>[2x]MPIITDVYAREVLDSRGNPTVEVEVLTESGAFGRALVPSGASTGEHEAVELRDGDKSRYLGKGVTKAVENVNEIIAPEIIEGEFSVLDQVSIDKMMIALDGTPNKGKLGANAILGVSIAVARAAADLLGQPLYKYLGGFNGKQLPVPMMNIVNGGSHSDAPIAFQEFMILPVGATTFKESLRWGTEIFHNLKSILSKRGLETAVGDEGGFAPKFEGTEDAVETIIQAIEAAGYKPGEEVFLGFDCASSEFYENGVYDYSKFEGEHGAKRTAAEQVDYLEQLVDKYPIITIEDGMDENDWDGWKQLTERIGDRVQLVGDDLFVTNTEILAKGIENGIGNSILIKVNQIGTLTETFDAIEMAQKAGYTAVVSHRSGETEDTTIADIAVATNAGQIKTGSLSRTDRIAKYNQLLRIEDELFETAKYDGIKSFYNLDKLEHHHHHH

Enolase is a glycolytic enzyme that requires a divalent metal ion (optimally Mg2+) bound in the active site to catalyze the dehydration of 2-phosphoglycerate (2-PG) to phosphoenolpyruvate (PEP), as well as the reverse reaction in the gluconeogenesis pathway. Interestingly, enolase has been identified on the cell surface of S. aureus, enhancing the staphylokinase activation of plasminogen. The Sa_enolase monomer has two distinct domains, a small N-terminal domain (residues 1–137) and a large C-terminal barrel domain (residues 149–434), connected by a linker region (residues 138–148). Biochemical and structural studies indicate that the octameric form of Sa_enolase is enzymatically active in vitro and likely also in vivo, while the dimeric form is catalytically inactive and may be involved in other biological processes.

The multiple functions of Sa_enolase encouraged further exploration, leading to determination of the crystal structure of Sa_enolase at 2.45 Å resolution. The non-ligand-bound Sa_enolase crystals belonged to space group P4212 and contained two monomers forming a single homodimer in the asymmetric unit. Structure alignment indicates that the two monomers are nearly identical, with a root-mean-square deviation (r.m.s.d.) of 0.2 Å for all Cα atoms. The monomer–monomer interface is vast and has a buried surface area of 1747 Å2. The dimer–dimer interfaces within the octamer form along the outer edges of neighbouring butterfly-like dimers and result in a buried surface area of ∼1287 Å2. Structural comparison of non-ligand-bound Sa_enolase with yeast enolase reveals that the non-ligand-bound Sa_enolase presented here assumes a conformation similar to the ‘open’ conformation of yeast enolase. Superimposition of the non-ligand-bound and PEP-bound structures of Sa_enolase reveals that conformational changes occur following ligand binding. The primary difference involves the orientation of L1, with residues 36–44 moving approximately 9.5 Å towards the centre of the active site in order to cover the catalytic pocket.> MSTPRKAAGNNENTEVSEIRTPFRE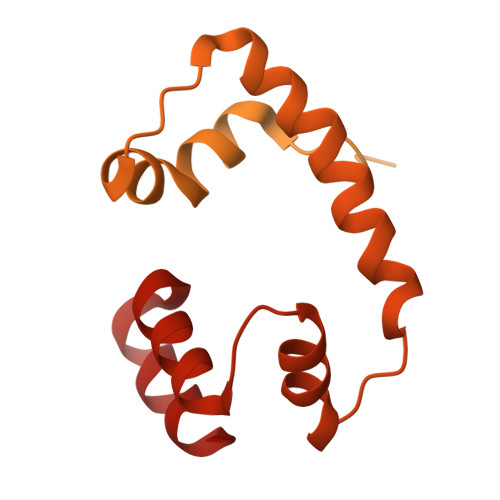RALEEQRLKDEVLIRNTPGYRKLLSASTKSHDILNKDPNEVRSFLQDLSQVLARKSQGNDTTTNKTQARNLIDELAYEESQPEENELLRSRSEKLTDNNIGNETQPDYTSLSQTVFAKLQERDKGLKSRKIDPIIIQDVPTTGHEDELTVHSPDKANSISMEVLRTSPSIGMDQVDEPPVRDPVPISITQQEEPLSEDLPSDDKEETEEAENEDYSFENTSDENLDDIGNDPIRLNVPAVRRSSIKPLQIMDLKHLTRQFLNENRIILPKQTWSTIQEESLNIMDFLKQKIGTLQKQELVDSFIDMGIINNVDDMFELAHELLPLELQSRIESYLFENLYFQ N-{1-[cis-4-(hydroxymethyl)cyclohexyl]-5-(piperidin-1-ylmethyl)-1H-benzimidazol-2-yl}-3-(prop-2-en-1-ylsulfamoyl)benzamide 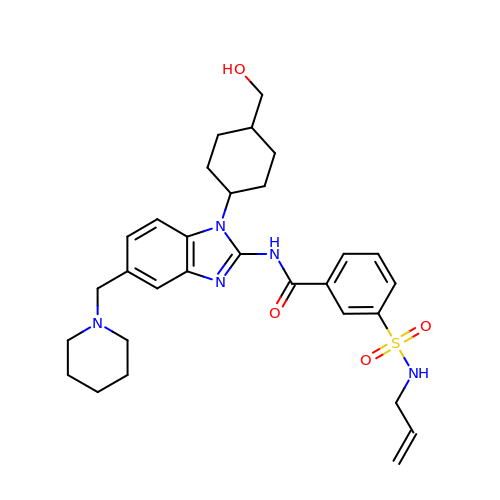| C30 H39 N5 O4 S | LWJAHJMKAARBCO-WZJNIGMMSA-N>[2x]GPHMVVAGIDPGITHL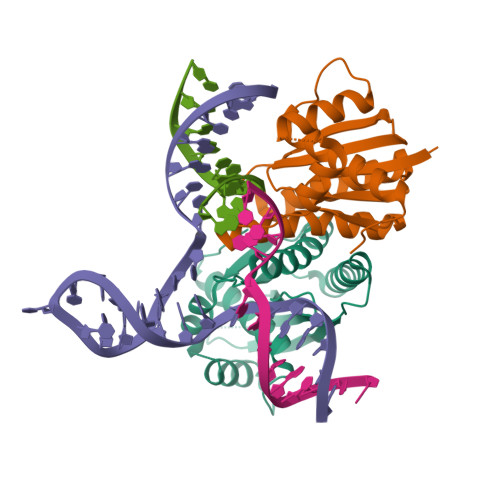GLGVVAVEGKGALKARLLHGEVVKTSPQEPAKERVGRIHARVLEVLHRFRPEAVAVQEQFFYRQNELAYKVGWALGAVLVAAFEAGVPVYAYGPMQVKQALAGHGHAAKEEVALMVRGILGLKEAPRPSHLADALAIALTHAFYARMGTAKPL>[2x]MEGMKGAVLITGASRGIGEATARLLHA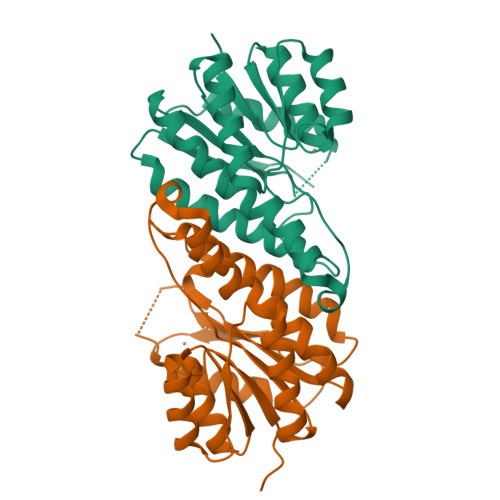KGYRVGLMARDEKRLQALAAELEGALPLPGDVREEGDWARAVAAMEEAFGELSALVNNAGVGVMKPVHELTLEEWRLVLDTNLTGAFLGIRHAVPALLRRGGGTIVNVGSLAGKNPFKGGAAYNASKFGLLGLAGAAMLDLREANVRVVNVLPGSVDTGFAGNTPGQAWKLKPEDVAQAVLFALEMPGHAMVSEIELRPTRPTSGPR>[13x]MHRSTGIGVSRWLGGLLGVALALPALALPQGCIELLAQAPRVDVVQGQQRDLRLAVPIERLAIGDPKIADVQLLDRRGFLVTGKEQGSTSLLIWTGCSPEPLRSLVEVEGRGSVDTRGAPAFTVGAAEELPNQVQTDIRFVEVSRSKLKQASTSFVRRGGNLWVLGAPGSLGDIKVNADGSGLGGTFGTGSSGFNLIFGGGKWLSFMNALEGSGFAYTLARPSLVAMSGQSASFLAGGEFPIPVPNGTNDNVTIEYKEFGIRLTLTPTVMNNRRIALKVAPEVSELDYSAGIQSGGVAVPALRVRRTDTSVMLADGESFVISGLTSSNSVSNVDKFPWLGDIPILGAFFRSTKLDKDDRELLMIVTPHLVQPLAADAQLPDLPGEGLRHYDPGFSRLYFLERGEYDGQQNDTGLSDSAW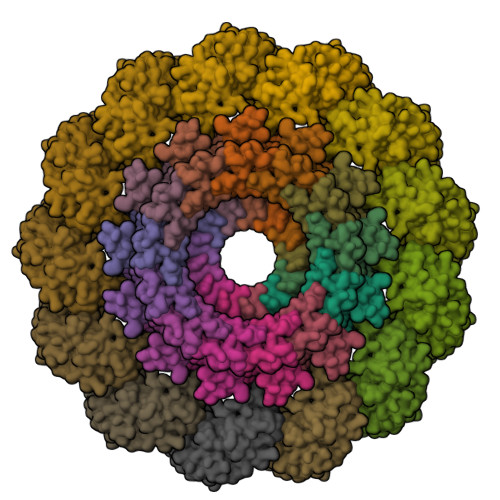SHPQFEK;>MKALIGIGLCAALLGGCAALPGRDGPRECSQQLGQEQELQMNMVRDMIREGRLHAALANLESMPPGLLDVREERALILRRIGDPRARAEYQALLETCKAPEAHHGLGLLALRNGDSARAVLELREAARLRPTESRFRNDLGVALLKRGDRVGARFEFITALELQQGGKLPATNLLGLLYLQGDREDAQRLIERLQLDARDIRAAEARARSWGAVPTPGAAPASDDPLAELPAEANMHTAMANEAPGSDYKDDDDK[13x]(2S)-2-[3-(AMINOMETHYL)PHENYL]-3-[(R)-{(1R)-1-[(BIPHENYL-4-YLSULFONYL)AMINO]-2-METHYLPROPYL}(HYDROXY)PHOSPHORYL]PROPANOIC ACID 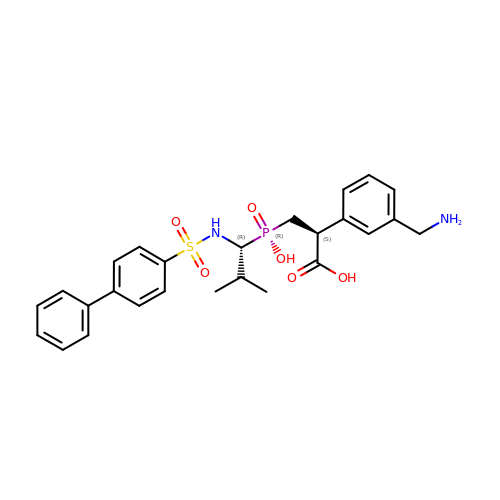| C26 H31 N2 O6 P S | KEOUUUFVAPIYKJ-LOSJGSFVSA-N> MITNSGKFGVVVVGVGRAGSVRLRDLKDPRSAAFLNLIGFVSRRELGSLDEVRQISLEDALRSQEIDVAYICSESSSHEDYIRQFLQAGKHVLVEYPMTLSFAAAQELWELAAQKGRVLHEEHVELLMEEFEFLRREVLGKELLKGSLRFTASPLEEERFGFPAFSGISRLTWLVSLFGELSLISATLEERKEDQ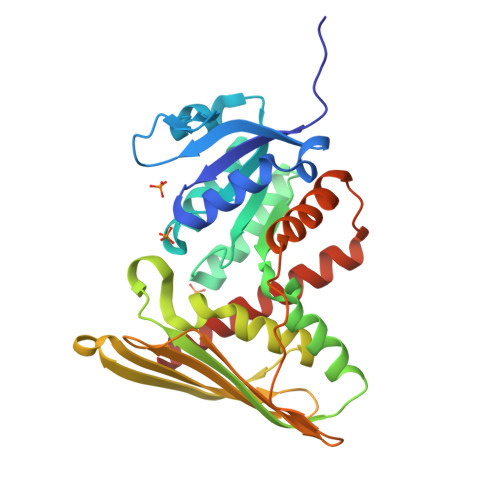YMKMTVQLETQNKGLLSWIEEKGPGLKRNRYVNFQFTSGSLEEVPSVGVNKNIFLKDQDIFVQKLLDQVSAEDLAAEKKRIMHCLGLASDIQKLCHQKK>[2x]MGHHHHHHHHHHSSGHIDDDDKHMPAHASPFNAPSSASRAGAARLGTSRRFAPFVLAALAILMGAMSVVALCVGAYRIPLAEAWAALSGDPAAQQARAVLLDIRAPRVVLALLVGGGFGATGAAMQALFRNPLADPGLVGVSSGAALGATTLIVLGPALFAAHASAAALPVAAFAGGLAVAALVYRLAASRGRLALPLLLLAGIAINALVGAAIGLLTFVADDAQLRSLTFWSLGSLGGAQWPTLAAVAPCVALGGVLLVRERDALNALQLGETEALHLGVPVQRLKRRVLVAVALAVGALVSCAGIIGFIGLVAPHCVRLACGPDQRIVLPGAALLGALLTLAADLAARTVAAPADIPLGVLTALLGAPFFLALLWKNRGALGG;>MLTAHHLDVARRHGTILRDLSLSIEPGRVTALLGRNGAGKSTLLKTFAGELTGSVAPHGVRVTGDVTLNGEPLARIDAPRLACLRAVLPQAAQPAFPFSVDEIVLLGRYPHARRSGATSHRDRDIAWRALERAGADALVGRDVTTLSGGELARVQFARVLAQLWPDHDTTEPGPRYLLLDEPTAALDLAHQHRLLDTVRAVAREWQLGVLAIVHDPNLAARHADAIAMLADGTIVAHGAPRDVMTPAHIAQCYGFAVKMVETGDGTPPVMVPA[2x]

Most pathogenic Gram-negative bacteria transport haem across the plasma membrane using an ATP-dependent active transport system, the ATP-binding cassette (ABC) transporter system. Here we describe the structures of the type II haem importer system (BhuUV-T) from the Gram-negative pathogen Burkholderia cenocepacia. BhuUV-T is a close orthologue of HmuUV-T910, which is a complex of BhuU (TMD), BhuV (NBD) and BhuT (PBP). We successfully characterized the structures of the ABC haem importer, the Bhu system from Burkholderia cenocepacia, and showed that both BhuUV-T and BhuUV adopt an inward-facing conformation in which the periplasmic gate of the haem-translocating channel is closed and the cytoplasmic gate is open.

The crystal structures of BhuUV-T and BhuUV were determined in the nucleotide-free form at 3.2 and 2.8 Å resolution, respectively. The structure of BhuUV consists of two TMDs (BhuU) and two NBDs (BhuV), while BhuUV-T is a heteropentamer complex comprising two TMDs, two NBDs and one PBP (BhuT). The structural characteristics of the channel, in which the periplasmic gate is closed and the cytoplasmic gate is open, allowed assignment of the observed structures of BhuUV-T and BhuUV to the inward-facing conformation. The corresponding region of BhuUV and BhuUV-T is located in the middle of the haem-transporting channel. L177, L178 and I181 create a hydrophobic patch and the cytoplasmic gate is open, as shown in Fig. 2b,e. The diameter of the gate is 13 Å (L177-L177 distance) and is the narrowest part of the channel, but the gate is wide enough for the haem (∼10 Å) to pass through. Inspection of the superposition of the two structures revealed that the dissociation of BhuT shows a slight change in the relative orientation of BhuU (∼2° along the axis perpendicular to the twofold dimer axis). However, the shift of the coupling helices and BhuV was also small (∼0.5 Å). We concluded that these small structural effects of BhuT-binding are consistent with the small effect of BhuT on ATPase activity. Although we should interpret the structures in detergent micelles carefully, our structural analysis showed that, in the absence of ATP, BhuUV without BhuT is still in the inward-facing conformation, indicating that BhuT dissociation is not a critical factor that imposes the conformational state from the inward- to the outward-facing conformation and initializes the haem-transport reaction. Turning next to the TMD–NBD complex of type II ABC transporter in the nucleotide-free form, both BhuUV and MolAB4 (33% amino-acid identity in TMD) adopt similar inward-facing conformations (rmsd of 1.1 Å for 205 Cα atoms in TM helices), whereas another haem importer, HmuUV (45% amino-acid identity in TMD; r.m.s.d. of 1.7 Å for 185 Cα atoms) and BtuCD (37% amino-acid identity in TMD; rmsd of 1.9 Å for 191 Cα atoms) are in the outward-facing conformation.>MSLEIQDSEVDIVIAALQPNLTTFFEAWRPFFSRFHIIVVKDPDMAEE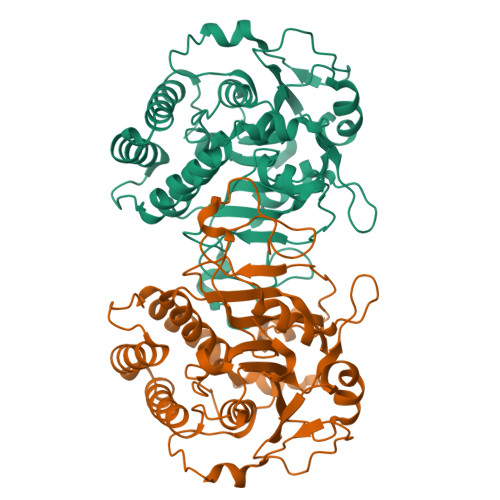LQIPTGFDLKVYTKSDMGVLGATSIDFSGHSCRYFGYLVSRKKYVISIDDNCLPAKDNGGLTVDAVAQHMSNLKTPATPFFFNTLYDPFRKGADFVRGYPFSLREGVECMLSCGLWLHNADYDPMTHVVKRNQRNTTYVDAVMTVPLGAMMPVSGINVAFNREVLGPVMFPALRLRKEGKHRWDTLEDVWNGLCAKVVCDRLRYGVKTGLPYVMRSDAEAGKALESLKEWEGVKVMDVVLPFFESLKLSSTSVTVEDCVKELTSIVKEKLGPQNAIFAKAADAMEEWTKLWKSHGAQSA[2x]>MTAEEMKATESGAQSAPLPMEGVDISPKQDEGVLKVIKREGTGTEMPMIGDRVFVHYTGWLLDGTKFDSSLDRKDKFSFDLGKGEVIKAWDIA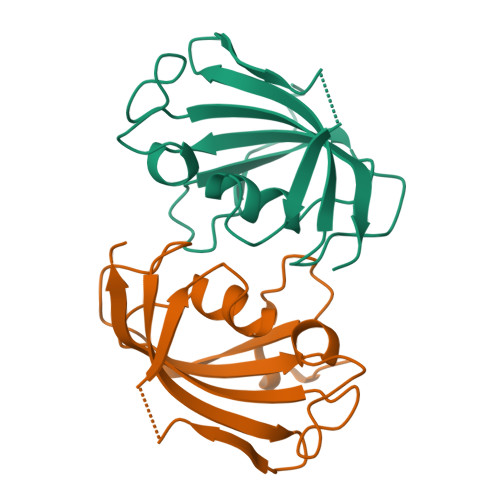IATMKVGEVCHITCKPEYAYGSAGSPPKIPPNATLVFEVELFEFKGE[2x]> QYAPQTQSGRTSIVHLFEWRWVDIALECERYLGPKGFGGVQVSPPNENVVVTNPSRPWWERYQPVSYKLCTRSGNENEFRDMVTRCNNVGVRIYVDAVINHMCGSGAAAGTGTTCGSYCNPGSREFPAVPYSAWDFNDGKCKTASGGIESYNDPYQVRDCQLVGLLDLALEKDYVRSMIADYLNKLID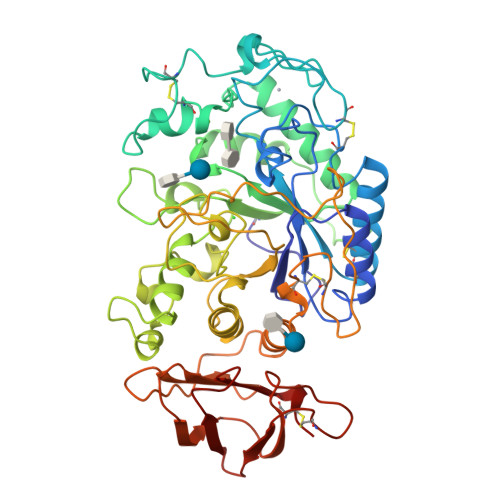IGVAGFRIDASKHMWPGDIKAVLDKLHNLNTNWFPAGSRPFIFQEVIDLGGEAIKSSEYFGNGRVTEFKYGAKLGTVVRKWSGEKMSYLKNWGEGWGFMPSDRALVFVDNHDNQRGHGAGGSSILTFWDARLYKIAVGFMLAHPYGFTRVMSSYRWARNFVNGEDVNDWIGPPNNNGVIKEVTINADTTCGNDWVCEHRWREIRNMVWFRNVVDGEPFANWWDNGSNQVAFGRGNRGFIVFNNDDWQLSSTLQTGLPGGTYCDVISGDKVGNSCTGIKVYVSSDGTAQFSISNSAEDPFIAIHAESKL Contrasting with Enterobacteria, members of the dominant genus Bacteroides often encode several BtuB vitamin B12 outer membrane transporters together with a conserved array of surface-exposed B12-binding lipoproteins. Here we show that the BtuB transporters from Bacteroides thetaiotaomicron form stable, pedal bin-like complexes with surface-exposed BtuG lipoprotein lids, which bind B12 with high affinities. Closing of the BtuG lid following B12 capture causes destabilisation of the bound B12 by a conserved BtuB extracellular loop, causing translocation of the vitamin to BtuB and subsequent transport. We propose that TonB-dependent, lipoprotein-assisted small molecule uptake is a general feature of Bacteroides spp. that is important for the success of this genus in colonising the human gut.

However, BtuB3G3 incubated with excess CNCbl in the mild detergent Lauryl Maltose Neopentyl Glycol (LMNG) eluted as a single peak and had a pink colour after SEC, suggesting the presence of bound CNCbl. We determined the structure of this complex by cryo-EM. Data analysis produced maps of sufficient quality to build two slightly different models, named state 1 and state 2. Both states show density for a CNCbl molecule bound to BtuG3. In state 2, while density for the tip of EL8 is absent, the visible part at the base (green) occupies an intermediate position between that in the BtuB2G2 apo structure (yellow) and state 1 in BtuB3G3-CNCbl (wheat). Moreover, state 2 density for CNCbl shows a different conformation for the vitamin. These observations suggest that, after ligand capture by BtuG3, EL8 in the closed complex is poised to move inwards and destabilises the vitamin in its BtuG3 binding pocket, perhaps acting like a spring-loaded hinge.

> MSGQQHSSDNKNWAEKGIVIREVEILGKRPMKDIGVQQTRFDSLVLKENIALSMADILTFNSSIFVKSYGRATLSTVSFRGTSASHTQVTWNGMRINNPMLGMTDFSMIPSYFIDDASLLHGTSSVNMAGGGLGGLVKLSTVPAHQEGFGMQYVQGIGSFSTFDEFLQLKYGDKHWQISTRAVYQSSPNDYKYRNHDKKENIYDDKYNIIEQYYPIERNRSGAYKDLHILQEVYYNTGKGDRFGLNAWYTDSNRELALLTTDQGDLMDFENRQREHTLRSVLSWDHTRENWKVSARGGYVHTWLAYDYKRDLGNGIMATMTRSRSKVNTFYGQLDGEYFFSDKLLLTAGVSAHQHLVNSLDKDLNKDDNKNDKYGQGRKNDSIVYFDKGRIELSGNVSLKWQPVNRLGMSLVLRGEMFGTKWAPVIPAFFVDYVLSKRGNIMAKASITRNYRFPTLNDLYFLPGGNPALNNESGFTYETGLSFSVDKDNVYTLSGSASWFDQHINDWIIWLPTSKGFYSPVNLKKVHAYGVEVQADYAVAIDKAWKLGLNGTFAWTPSINEGEPTSKADQSVGKQLPYIPEYSATLSGRLTYRSWGLLYKWCYYSERYTMTSNAVSYTGHLPPYLMSNVTLEKGFSLRWADLSLKGTVNNLFDEEYLSVLSRPMPGINFEFFIGITPKWGKKKKGGGHHHHHH;> MKRILLSVLFIVFCLTAFVGCMKWDYGKMEPFRATGDGLFIMNEGNFQYGNATLSYYDPETKKVENEIFYRANAMKLGDVAQSMIVRDTIGWVVVNNSHVIFAISTNTFKEVGRITGLTSPRYIHFISDEKAYITQIWDYRIFIVNPKTYQITGYIECPDMTMETGSTEQMVQYGKYVYVNCWSYQNRILKIDTTTDKVVDQLTVGIQPTSLVMDKNFKMWTITDGGYKGSPYGYEEPSLYRIDAETFKIEKQFKFQLGDAPSEVQLNGAGDELYWINKDIWRMSVDEERVPVRPFLKYRDTKYYGLTVSPKNGDVYVADAIDYQQQGMIYRYTEDGELVDEFYVGIIPGAFCWK4-methyl-~{N}-oxidanyl-3-[(phenylmethyl)amino]benzamide | C15 H16 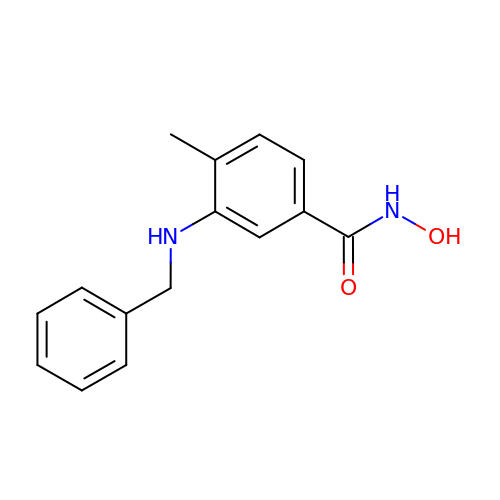N2 O2 | PZBARTUEWCQNSN-UHFFFAOYSA-N1H-pyrrolo[3,2-b]pyridin-6-ylmethanol | C8 H8 N2 O | 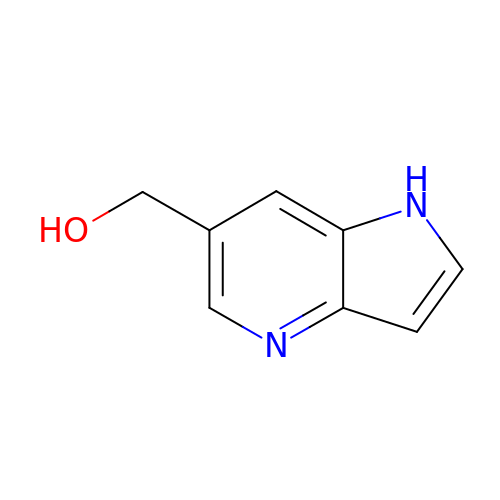PHEOXCPRDIGDAZ-UHFFFAOYSA-N3-(PROP-2-ENE-1-SULFINYL)-PROPENE-1-THIOL 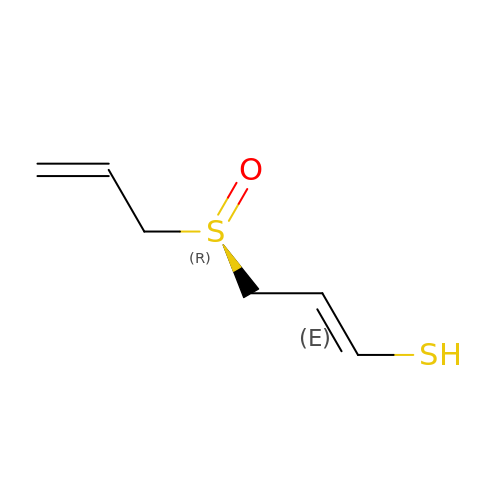| C6 H10 O S2 | HSVQDVSVQIMRSS-CDAZIORVSA-N>[4x]TEKKYIVALDQGTTSSRAVVM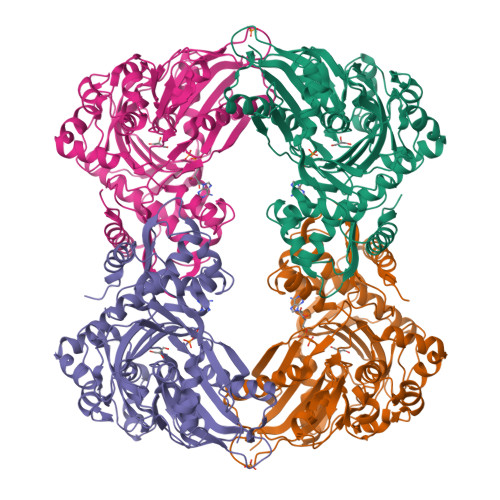DHDANIISVSQREFEQIYPKPGWVEHDPMEIWATQSSTLVEVLAKADISSDQIAAIGITNQRETTIVWEKETGKPIYNAIVWQCRRTAEICEHLKRDGLEDYIRSNTGLVIDPYFSGTKVKWILDHVEGSRERARRGELLFGTVDTWLIWKMTQGRVHVTDYTNASRTMLFNIHTLDWDDKMLEVLDIPREMLPEVRRSSEVYGQTNIGGKGGTRIPISGIAGDQQAALFGQLCVKEGMAKNTYGTGCFMLMNTGEKAVKSENGLLTTIACGPTGEVNYALEGAVFMAGASIQWLRDEMKLINDAYDSEYFATKVQNTNGVYVVPAFTGLGAPYWDPYARGAIFGLTRGVNANHIIRATLESIAYQTRDVLEAMQADSGIRLHALRVDGGAVANNFLMQFQSDILGTRVERPEVREVTALGAAYLAGLAVGFWQNLDELQEKAVIEREFRPGIETTERNYRYAGWKKAVKRAMAWEEHDE>GSDYENDDECWSVLEGFRVTLTSVIDPSRITPYLRQCKVLNPDDEEQVLSDPNLVIRKRKVGVLLDILQRTGHKGYVAFLESLE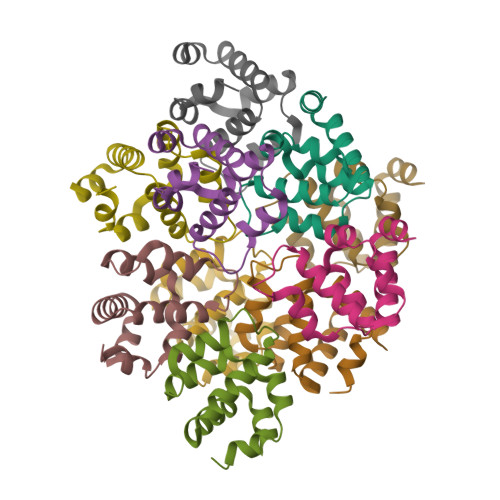LYYPQLYKKVTGKEPARVFSMIEDASGESGLTQLLMTEVMKLQKKVQDLTALLSSKDDFIKELRVKDS[10x]> MRDHRKIGKQLDLYHMQEEAPGMVFWHNDGWTIFRELEVFVRSKLKEYQYQEVKGPFMMDRVLWEKTGHWDNYKDAMFTTSSENREYCIKPMNCPGHVQIFNQGLKSYRDLPLRMAEFGSCHRNEPSGSLHGLMRVRGFTQDDAHIFCTEEQIRDEVNGCIRLVYDMYSTFGFEKIVVKLSTRPEKRIGSDEMWDRAEADLAVALEENNIPFEYQLGEGAFRGPKIEFTLYDCLDRAWQCGTVQLDFSLPSRLSASYVGEDNERKVPVMIHRAILGSMERFIGILTEEFAGFFPTWLAPVQVVIMNITDSQSEYVNELTQKLSNAGIRVKADLRNEKIGFKIREHTLRRVPYMLVCGDKEVESGKVAVRTRRGKDLGSMDVNEVIEKLQQEIRSRSLKQLEELEHHHHHH

Aminoacyl-tRNA synthetases (AARSs), a family of essential protein synthesis enzymes, are attractive targets for drug development. Here we present five unusual crystal structures showing that threonyl-tRNA synthetase (ThrRS) is covalently inhibited by a natural product, obafluorin (OB). OB contains a β-lactone ring with a 2,3-dihydroxybenzamidyl moiety attached to the α position and a 4-nitrobenzyl moiety attached to the β position. When ThrRS catalyzes tRNA aminoacylation, the Zn2+ ion recognizes and binds l-threonine, assisting in the l-threonine activation reaction.

Because the length of the side chain of arginine is also not that different from tyrosine, we designed a ThrRS_Y462R mutant. Although the guanidinium group of arginine has less inclination for the donation of electron density due to resonance, we wondered if the β-lactone could covalently modify arginine when it was properly positioned. Not surprisingly, OB only increased the Tm of ThrRS_Y462R by 6.5 °C in the TSA experiment, which was higher than that of ThrRS_Y462F but significantly lower than that of ThrRS_WT or ThrRS_Y462K. This result suggests that Arg462 could not react with β-lactone during the relatively short period of time in the TSA experiment. When we cocrystallized ThrRS_Y462R with OB and ATP, we expected that ATP would exclude OB from the active pocket of ThrRS_Y462R if OB failed to form a covalent bond with the enzyme, as we have observed in the ThrRS_Y462F structure. However, the result was surprising in that Arg462 actually formed a covalent bond with OB, while no ATP was observed in the pocket. This result indicates that although the activity of the arginine mutant is reduced, it can still react with β-lactone to form a covalent bond over a longer period of time, as it takes approximately 24 h for crystal growth. Another discovery in this study is that β-lactone can modify arginine, although it is not highly reactive.>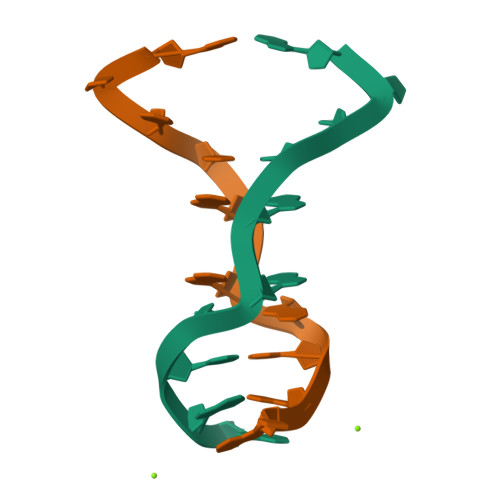ACTCGGACGAT[4x]The glutaminase enzymes GAC and GLS2 catalyze the hydrolysis of glutamine to glutamate, satisfying the ‘glutamine addiction’ of cancer cells. All glutaminase enzymes share a catalytic domain containing identical active site residues and a conserved mechanism for hydrolyzing glutamine to glutamate. Here we demonstrate that the ability of GAC and GLS2 to form filaments is directly coupled to their catalytic activity and present their cryo-EM structures which provide a view of the conformational states essential for catalysis. Filament formation guides an ‘activation loop’ to assume a specific conformation that works together with a ‘lid’ to close over the active site and position glutamine for nucleophilic attack by an essential serine.

Several high-resolution X-ray structures for KGA and GAC have been reported; however, thus far, there has not been a structural determination for the full-length apo-GLS2 protein. Therefore, we obtained a cryo-EM structure for wild-type, full-length GLS2. Figure 1a, b show the 3.1 Å structure of the human apo-GLS2 tetramer and the relative positions of the key regions for catalytic activity (i.e., the ‘activation loop’, the catalytic site, and the ‘lid loop’ that opens and closes over the catalytic domain). The stretch of residues Gly248-Glu258, which has been shown to play an essential role in catalysis and thus referred to as the ‘activation loop'23,34, is disordered and flexible in the GLS2 structure. In addition, residues Tyr182-Lys188 in GLS2, which correspond to a loop in KGA and GAC forming a ‘lid’ that needs to close over bound substrates for catalysis to occur, are also flexible like the activation loops in the GLS2 structure. The C-terminal region of GLS2 contains an ankyrin repeat motif consisting of three pairs of helical bundles located on the distal ends of the tetramer, which is absent in GAC. Each GLS2 dimer within a tetrameric unit shares an ankyrin repeat bundle connected to the catalytic domain through a flexible linker. Interestingly, the ankyrin repeats asymmetrically occupy the area between the N-terminus of adjacent monomeric units within a dimer, showing a preferential association for one monomer over the other. However, within the GLS2 structure, the ankyrin repeats appear to hinder this movement and thereby may prevent the activation loops from adopting the positions necessary for maximal catalytic capability.

>MRSMKALQKALSRAGSHCGRGGWGHPSRSPLLGGGVRHHLSEAAAQGRETPHSHQPQHQDHDSSESGMLSRLGDLLFYTIAEGQERIPIHKFTTALKATGLQTSDPRLRDCMSEMHRVVQESSSGGLLDRDLFRKCVSSNIVLLTQAFRKKFVIPDFEEFTGHVDRIFEDVKELTGGKVAAYIPQLAKSNPDLWGVSLCTVDGQRHSVGHTKIPFCLQSCVKPLTYAISISTLGTDYVHKFVGKEPSGLRYNKLSLNEEGIPHNPMVNAGAIVVSSLIKMDCNKAEKFDFVLQYLNKMAGNEYMGFSNATFQSEKETGDRNYAIGYYLKEKKCFPKGVDMMAALDLYFQLCSVEVTCESGSVMAATLANGGICPITGESVLSAEAVRNTLSLMHSCGMYDFSGQFAFHVGLPAKSAVSGAILLVVPNVMGMMCLSPPLDKLGNSHRGTSFCQKLVSLFNFHNYDNLRHCARKLDPRREGAEIRNKTVVNLLFAAYSGDVSALRRFALSAMDMEQKDYDSRTALHVAAAEGHIEVVKFLIEACKVNPFAKDRWGNIPLDDAVQFNHLEVVKLLQDYQDSYTLSETQAEAAAEALSKENLESMV[4x]>FDRADILYNIRQTSRPDVIPTQRDRPVAVSVSLKFINILEVNEITNEVDVVFWQQTTWSDRTLAWNSSHSPDQVSVPISSLWVPDLAAYNAISKPEVLTPQLARVVSDGEVLYMPSIRQRFSCDVSGVDTESGATCRIKIGSWTHHSREISVDPTTENSDDSEYFSQYSRFEILDVTQKKNSVTYSCC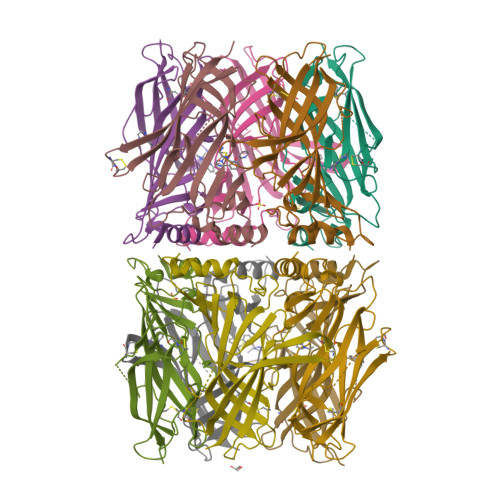PEAYEDVEVSLNFRKKGR[10x]>ARPCIPKSFGYSSVVCVCNATYCDSFDPPTFPALGTFSRYESTRSGRRMELSMGPIQANHTGTGLLLTLQPEQKFQKVKGFGGAMTDAAALNILALSPPAQNLLLKSYFSEEGIGYNIIRVPMASCDFSIRTYTYADTPDDFQLHNFSLPEEDTKLKIPLIHRALQLAQRPVSLLASPWTSPTWLKTNGAVNGKGSLKGQPGDIYHQTWARYFVKFLDAYAEHKLQFWAVTAENEPSAGLLSGYPFQCLGFTPEHQRDFIARDLGPTLANSTHHNVRLLMLDDQRLLLPHWAKVVLTDPEAAKYVHGIAVHWYLDFLAPAKATLGETHRLFPNTMLFASEACVGSKFWEQSVRLGSWDRGMQYSHSIITNLLYHVVGWTDWNLALNPEGGPNWVRNFVDSPIIVDITKDTFYKQPMFYHLGHFSKFIPEGSQRVGLVASQKNDLDAVALMHPDGSAVVVVLNRSSKDVPLTIKDPAVGFLETISPGYSIHTYLWRRQ[2x]

Gaucher disease (GD) is the most common lysosomal storage disorder which is caused by inherited deficiencies in β‐glucocerebrosidase (glucosylceramidase, GCase, GBA, EC 3.2.1.45). GBA is primarily responsible for catalyzing the degradation of GlcCer by hydrolytic cleavage of the β‐glucose moiety from the aglycone to yield free ceramide and glucose. This is achieved with retention of β‐anomeric stereochemistry of the released glucose unit through a Koshland double displacement mechanism using Glu340 as the catalytic nucleophile and Glu235 as the catalytic acid‐base. Here, we report the design, synthesis, and structural analysis of a range of cyclophellitol epoxide and aziridine inactivators and activity‐based probes (ABPs) for human β‐glucocerebrosidase (GBA).

Therefore, to probe whether this holds true from a mechanistic inhibition point of view, a crystal structure rhGBA in complex with cyclophellitol aziridine 2 was obtained at 1.70 Å resolution to enable a detailed comparison with cyclophellitol epoxide 1. The electron density of the resulting co‐crystal structure unambiguously shows that 2 reacts with the enzymatic nucleophile of GBA (Glu340) through the aziridine warhead to form a covalent trans‐diaxial ring opened complex which is essentially identical to reacted cyclophellitol epoxide 1. Indeed, 2 forms a covalent complex in the 4C1 chair conformation with a covalent bond length of 1.46 Å to Glu340. The only notable difference between the complex of 2 and 1 lies in their hydrogen bonding networks, where a hydrogen bond is formed between the O6‐hydroxyl of 2 and Asn396, and the hydrogen bond to Tyr313 is lost, likely due to the “downwards” displacement of Tyr313 in complex with 2. The flexibility of Tyr313 has been reported previously and the “downwards” conformation observed in complex with 2 appears to preclude hydrogen bonding with the ring‐opened aziridine. Instead, the aziridine warhead forms a hydrogen bond to a nearby water molecule in the active site. Overall, this co‐crystal structure demonstrates the almost identical binding mode of cyclophellitol epoxides and aziridines, which supports their interchangeable use in the development of ABPs for GBA.> ADVPAGVQLADKQTLVRNN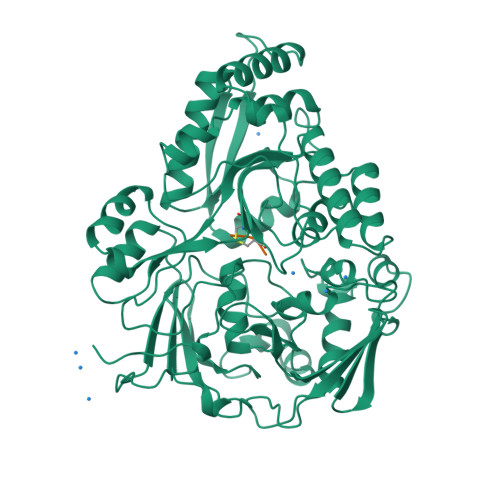GSEVQSLDPHKIEGVPESNVSRDLFEGLLISDVEGHPSPGVAEKWENKDFKVWTFHLRENAKWSDGTPVTAHDFVYSWQRLADPNTASPYASYLQYGHIANIDDIIAGKKPATDLGVKALDDHTFEVTLSEPVPYFYKLLVHPSVSPVPKSAVEKFGDKWTQPANIVTNGAYKLKNWVVNERIVLERNPQYWDNAKTVINQVTYLPISSEVTDVNRYRSGEIDMTYNNMPIELFQKLKKEIPNEVRVDPYLCTYYYEINNQKAPFNDVRVRTALKLALDRDIIVNKVKNQGDLPAYSYTPPYTDGAKLVEPEWFKWSQQKRNEEAKKLLAEAGFTADKPLTFDLLYNTSDLHKKLAIAVASIWKKNLGVNVNLENQEWKTFLDTRHQGTFDVARAGWCADYNEPTSFLNTMLSDSSNNTAHYKSPAFDKLIADTLKVADDTQRSELYAKAEQQLDKDSAIVPVYYYVNARLVKPWVGGYTGKDPLDNIYVKNLYIIKH;> KWK> GAKPYEKVRIYRMDGSYRSVELKHGNNTTVQQIMEGMRLSQETQQYFTIWICSENLSLQLKPYHKPLQHVRDWPEILAELTNLDPQRETPQLFLRRDVRLPLEVEKQIEDPLAILILFDEARYNLLKGFYTAPDAKLITLASLLLQIVYGNYESKKHKQGFLNEENLKSIVPVTKLKSKAPHWTNRILHEYKNLSTSEGVSKEMHHLQRMFLQNCWEIPTYGAAFFTGQIFTKASPSNHKVIPVYVGVNIKGLHLLNMETKALLISLKYGCFMWQLGDTDTCFQIHSMENKMSFIVHTKQAGLVVKLLMKLNGQLMPTERNS;> MREYKLVVL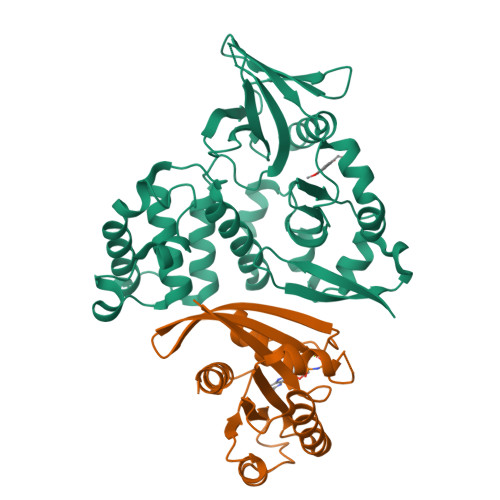GSGGVGKSALTVQFVQGIFVEKYDPTIEDSYRKQVEVDAQQCMLEILDTAGTEQFTAMRDLYMKNGQGFALVYSITAQSTFNDLQDLREQILRVKDTDDVPMILVGNKCDLEDERVVGKEQGQNLARQWNNCAFLESSAKSKINVNEIFYDLVRQINR> VSETLVENFLSRAALVSKRSFEYKDHTSSTAQTDKNFFKWTINTRSFVQLRRKLELFTYLRFDAEITILTTVAVNGSNNNTYVGLPDLTLQAMFVPTGALTPEKQDSFHWQSGSNASVFFKISDPPARMTIPFMCINSAYSVFYDGFAGFEKTGLYGINPADTIGNLCVRIVNEHQPVGFTVTVRVY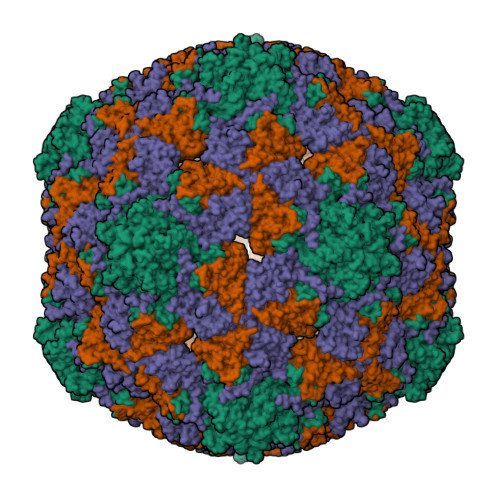MKPKHIKAWAPRPPRTLPYMSIANANYKG;> ANYCCAYGEWPNYLPDHEAVAIDKPTQPETATDRFYTLRSVKWEATSTGWWWKLPDALNNIGMFGQNVQHHYLYRSGFLIHVQCNATKFHQGALLVVAIPEHQRGAHNTTTSPGFDDIMKGEAGGTFNHPYVLDDGTSLACATIFPHQWINLRTNNSATIVLPWMNAAPMDFPLRHNQWTLAIIPVVPLGTRTMSSMVPITVSIAPMCCEFN;> GVPTYLLPGSGQFLTTDDHSSAPVLPCFNPTPEMHIPGQVRNMLEVVQVESMMEINNTESAVGMERLKVDISALTDVDQLLFNIPLDIQLDGPLRNTLVGNISRYYTHWSGSLEMTFMFCGSFMATGKLILCYTPPGGSCPTTRETAMLGTHIVWDFGLQSSITLIIPWISGSHYRMFNNDAKSTNANVGYVTCFMQTNLIVPSESSDTCSLIGFIAAKDDFSLRLMRDSPDIGQIDHLHGAEAAYQ>GPLGSCSSPQVEIPTTYSPEKIAQLQVYVNPIAVARDGMEKRLQGLIADQNWVDTQTYIHGPLG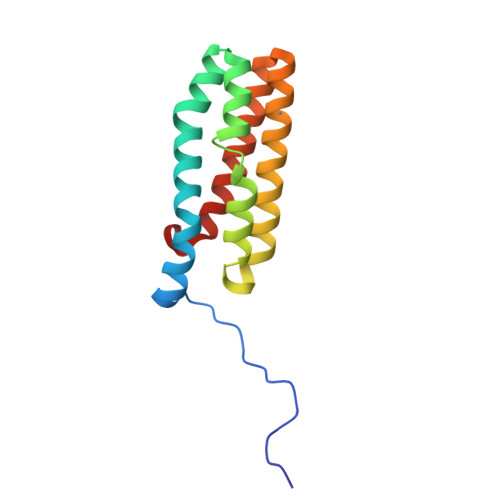QLRRDMLGLASSLLPKDQDKAKTLAKEVFGHLERLDAAAKDRNGSQAKIQYQEALADFDSFLNLLPQAS[2x]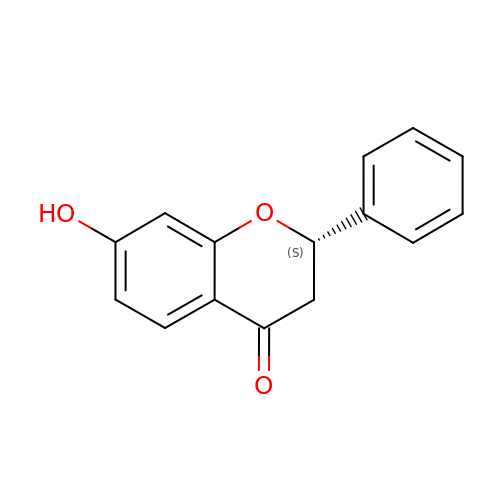7-HYDROXY-2-PHENYL-CHROMAN-4-ONE | C15 H12 O3 | SWAJPHCXKPCPQZ-AWEZNQCLSA-N> MASLLTETMPFKTTIEGTVNGHCFKCIGKGEGNPFEGTQEMKIEVIEGGPLPFAFHILSTSCMYGSKTFIKYVSGIPDYFKQSFPEGFTWERTTTYEDGGFLTAHQDTS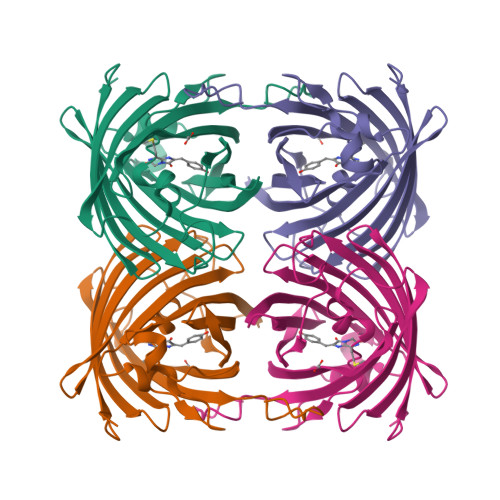LDGDCLVYKVKILGNNFPADGPVMQNKVGRWEPGTEIVYEVDGVLRGQSLMALKCPGGRHLTCHLHTTYRSKKPASALKMPGFHFEDHRIEIMEEVEKGKCYKQYEAAVGRYCDAAPSKLGHN>MSTGDFLTKGIELVQKAIDLDTATQYEEAYTAYYNGLDYLMLALKYEKNPKSKDLIRAKFTEYLNRAEQLKKHLESEEANAAKKSPSAGSGSNGGNKKISQEEGEDNGGEDNKKLRGALSSAILSEKPNVKWEDVAGLEGAKEALKEAVILPVKFPHLFKGNRKPTSGILLYGPPGTGKSYLAKAVATEANSTFFSVSSSDLVSKWMGESEKLVKQLFAMARENKPSIIFIDQVDALTGTRGEGESEASRRIKTELLVQMNGVGNDSQGVLVLGATNIPWQLDSAIRRRFERRIYIPLPDLAARTTMFEINVGDTPCVLTKEDYRTLGAMTEGYSGSDIAVVVKDALMQPIRKIQSATHFKDVSTEDDETRKLTPCSPGDDGAIEMSWTDIEADELKEPDLTIKDFLKAIKSTRPTVNEDDLLKQEQFTRDFGQEGN[6x];>MASNAARVVATAKDFDKVGLGIIGYYLQLYAVELILSEEDRSQEMTALATELLDTIEAFKKEIGGESEAEDSDKSLHVMNTLIHDQEKAKIYMLNFTMSLYNEKLKQLKDGPWDVMLKRSLWCCIDLFSCILHLWKENISETSTNSLQKRIKYCKIYLSKLAKGEIGSSDEKTLDYADFADDSEEIKDEDVDHQTSDLENNNNDKVEGLAPKDQTTSYEPVDEVPEFIDDADSVNEEEQTVDKN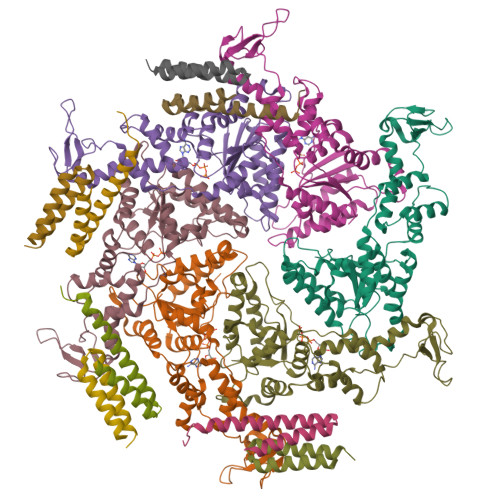EDAITKDEQQVVKKEVDLTRPSAPSEPAAAEHKSYTKDELTKIMDRASKIEQIQKLAKYAISALNYEDLPTAKDELTKALDLLNSI[8x]(3R,4S,5R,6R)-4-amino-3,5-dihydroxy-6-methyloxan-2-yl][hydroxy-[[(2R,3S,5R)-3-hydroxy-5-(5-methyl-2,4-dioxopyrimidin-1-yl)oxolan-2-yl]methoxy]phosphoryl] 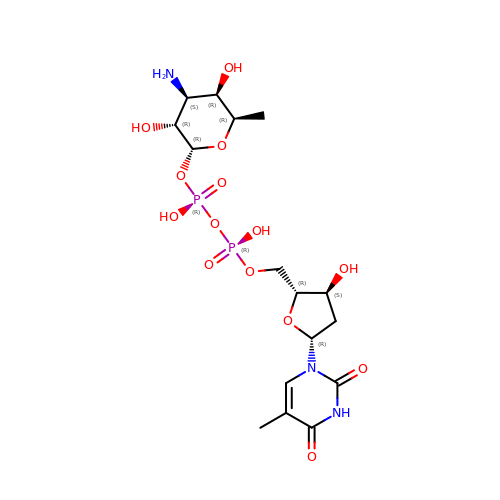hydrogen phosphate | C16 H27 N3 O14 P2 | KVYJLJOGNUNRJK-FQLHZTMTSA-N>[2x]MAPWKIEEVKTLKGLIKSKPVVAIVDMMDVPAPQLQEIRDKIRDKVKLRMSRNTLIIRALKEAAEELNNPKLAELANYVERGAAILVTDMNPFKLYKL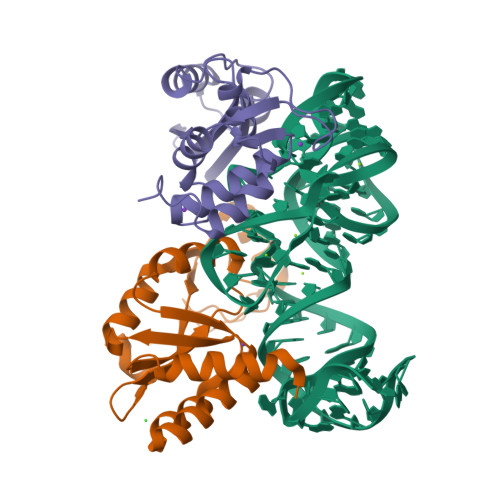LEENKSPAPVRGGQIAPCDIKVEKGSTGMPPGPFLGELKSVGIPAAIEKGKIAIKEDKVVVKKGEVVSPKLAAVLDRLGIKPIKVGLNILAVYEDGIIYTPDVLKVDEEKLLADI;>[2x]MAKEVVEVLVTGGRATAGPPLGPAIGPLGVNVMQVVKEINEKTKDYEGMQVPVKVIVDTETRKFEIEVGIPPTTALIKKELGIETAAHEPRHEVVGNLTLEQVIKIAKMKKDAMLSYTLKNAVKEVLGTCGSMGVTVEGKDPKEVQKEIDAGVYDEYFKEE> DPTVSKYNVTGNNGTCLLA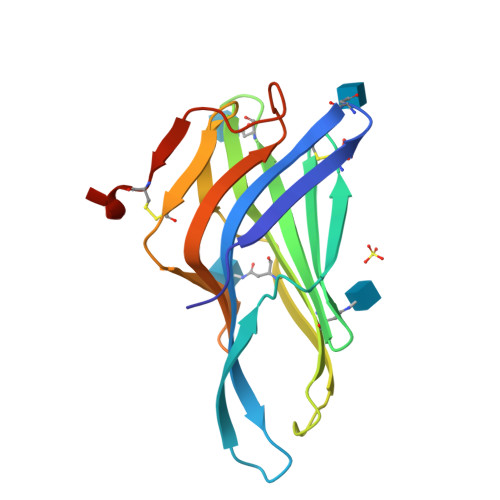SMALQLNITYLKKDNKTVTRAFNISPNDTSSGSCGINLVTLKVENKNRALELQFGMNASSSLFFLQGVRLNMTLPDALVPTFSISNHSLKALQATVGNSYKCNTEEHIFVSKMLSLNVFSVQVQAFKVDSDRFGSVEECVQDGNNGSSL> RADVKPVTVKLVDSQATMETRSLFAFMQEQRRHSIMFGHQHETTQGLTITRTDGTQSDTFNAVGDFAAVYGWDTLSIVAPKAEGDIVAQVKKAYARGGIITVSSHFDNPKTDTQKGVWPVGTSWDQTPAVVDSLPGGAYNPVLNGYLDQVAEWANNLKDEQGRLIPVIFRLYHANTGSWFWWGDKQSTPEQYKQLFRYSVEYLRDVKGVRNFLYA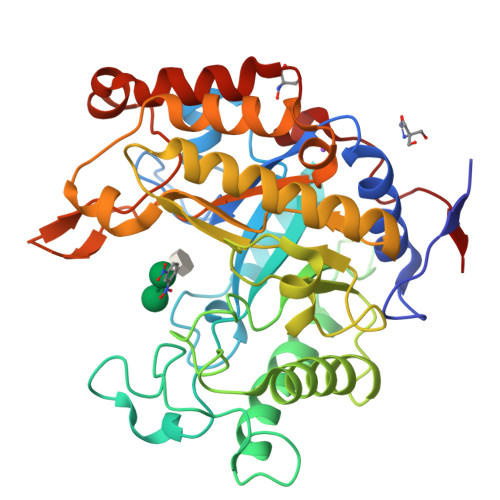YSPNNFWDVTEANYLERYPGDEWVDVLGFDTYGPVADNADWFRNVVANAALVARMAEARGKIPVISEIGIRAPDIEAGLYDNQWYRKLISGLKADPDAREIAFLLVWRNAPQGVPGPNGTQVPHYWVPANRPENINNGTLEDFQAFYADEFTAFNRDIEQVYQRPTLI>MPDFLGHAENPLREEEWARLNETVIQVARRSLVGRRILDIYGPLGAGVQTVPYDEFQGVSPGAVDIVGEQETAMVFTDARKFKTIPIIYKDFLLHWRDIEAARTHNMPLDVSAAAGAAALCAQQEDELIFYGDARLGYEGLMTANGRLTVPLGDWTSPGGGFQAIVEATRKLNEQGHFGPYAVVLSPRLYSQLHRGGEIETIRQLASDGVYQSNRLRGESGVVVSTGRENMDLAVSMDMVAAYLGASRMNHPFRVLEALLLR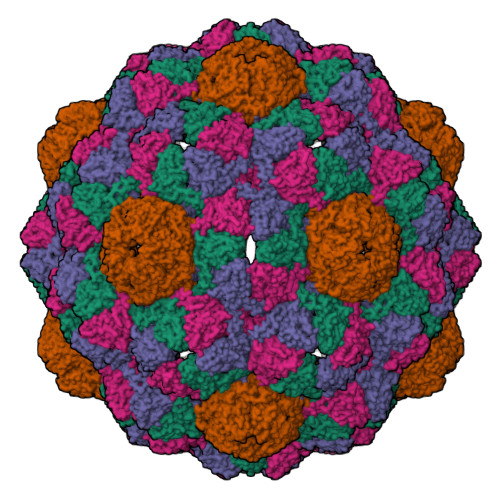IKHPDAICTLEGAGATERR[4x];>PEKRLTVGSLRR[4x]>MASNSPTFKHESYYATVNELTPVGTTI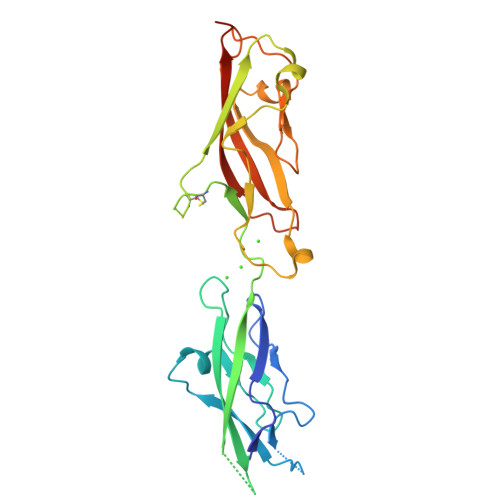FTGFSGDNGATDIDDGPNGQIEYVIQYNPDDPTSNDTFEIPLMLTGNIVLRKRLNYEDKTRYFVIIQANDRAQNLNERRTTTTTLTVDVLDGDDLGPMFLPCVLNPNTRDCRPLTYQAAIPELRTPEELNPIIVTPPIQAIDQDRNIQPPSDRPGILYSILVGTPEDYPRFFHMHPRTAELSLLEPVNRDFHQKFDLVIKAEQDNGHPLPAFAGLHIEILDENNLEHHHHHH[2x]> MSLGAKPFGEKKFIEIKGRRMAYIDEGTGDPILFQHGNPTSSYLWRNIMPHCAGLGRLIACDLIGM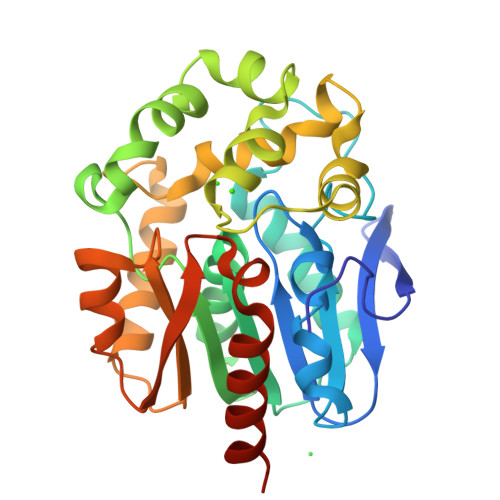GDSDKLDPSGPERYTYAEHRDYLDALWEALDLGDRVVLVVHDWGSVLGFDWARRHRERVQGIAYMEAVTMPLEWADFPEQDRDLFQAFRSQAGEELVLQDNVFVEQVLPGLILRPLSEAEMAAYREPFLAAGEARRPTLSWPRQIPIAGTPADVVAIARDYAGWLSESPIPKLFINAEPGHLTTGRMRDFCRTWPNQTEITVAGAHFIQEDSPDEIGAAIAAFVRRLRPAHHHHHH> MWHYTSINNDTRVALDPKPNQIRTITKPNTVPQLGTDYLYTFNSQRRSHTLRLLGPFQYFNFSETDRGHPLFRLPLKYPSKAIPADELIDNLHSWMRSVHLLHVRSEDNTLRYNWMLGVYARSTNYTTPVGQLVVNAPAILNYSNPQDAFNSVFVALGIDYIDIPITNSNIFDDSSTPYNVRIWHAPTMTEVNHILALMRKSTLVSTHSSWHWNVLHTFHYRSESDMIDHFAAKILEDWRQKEKLDKGALVEADRVIQRLIPLSSSTYVQRLAAIGALYPNEFTENVLDLSRLSTALLQLSDTYYQHANDQLRRLYRRMYNDSRTLYMTQRHQELLLAQITADPNILLYPYTYIFTTIPTSMNYISNTGQGRIKHSLTVTGATEHDTVADIVLGQTGEDVITISMVEPMSIAVEDMYGYVLDTPTRDIWPADEQIEQKGDAVALYDTKTSRALGMFNNTVRIDDLLSPLLSLVYRTYIKGDTMTMTQGSLDHLTLCAAVDSDITFVGNRMIAPLPEGYIPKPMHRNNSTMKMLSLYVALKKLENFATNSYLMAPDTSIILLGAEREPAVNILRRFNRNVSNVRIIGMGDRAVEPNIRVRVPFPIDKNISADFIICDINSYEDQSFESMFSETISVVTTCASAATRALVKINHPSEYMINSVIERLSQLGGVFYHTALLKTASQNPYSYETYIYITPIAAAVRFPFYSNSAMINRYMTAVADDEMPIIPSIHTVIKGHSNTYSPGLFCGCVDVQSAPLALSQLKSYCSEATTWRVDSDDNLVNIIARIDPARIALEFRTRSNTSAYHEYQRYVPNGLGFKVRKTREFRYMHREVTFIHKLMMYALIREQISLTENMTQVVSIGGRNLADISVVPLNMKYVVIDPATRIETLTQEKKNIEVQSRPFQFDAANMDLENNSIYLFIAVIMNEPNGAATPARMQMDKIRNVATAMLTRTNCVAYISFYEAGIITRLDQSTAHKTIRVEEGRLKVANYVPVDTLVEADVTLMLRDIGITHEIIRPSTPELIDACSNYGIRLGSTGGAVLDVFNHYSPVIKLVRS;>MHSTNNNSNKRNNEEKHKQPEIDSSANNGEGTSGTRAQTVGDTATEAGVRNETEAGASTRRQTDGTGLSGTNAKIATASSARQADVEKPADVTFTIENVDDVGIMQQKKPPTVVQSRTDVFNEQFANEALHPTTKVIFNGLDVNTEVQPLSDDFKQISDPKGYLTYSVKYEDQFTKKDKLRASEADDRIVGPTVNLFKYGAAVVNIDLNRDFFDTATGIDLTKGIPLVQDLLVPIGVTAGAEQSAEYVSGLLMVLFKVMTDNRLVIVGETTTPMSNTLSTVVNNVLRTTYHNNVGVNPALLRDFTQVNWLNRDITNMLQQAGTKYGLGLTETRLDYVRLVKTIVGHALNIDHFAASVLNINLRALMEANVTADDRIKALQAHSMISTQFHGPNQGALRPELAFDHDHIIRCLMLAAANYPRLEGIIVQINTGYVASANVIRPVSEKRYFPENLEQNQSAARLVSAVKARASEADISSIHLAIAREVSPMFNVHELKKIAESFEDPSSIVVVLEFILFALFFPTEFNRIKGDIQNVLLLFFSRWYPVEYGIFVQRGATYTINAAGEFEFSGRNEKWDQALYLSEHFPALFSDVPLAGANTIIAIMRLFTPQGFLRTDDLAIAANFPRASRNPQTYIPYTNQRGTVTNEFASRFRTIVATLANVVNERAVQDDMQKATRSCTKQWLRHLETQFDNIAVAHTDHLSVVYATMSNFMLNFTNNFSGNHATFKPDQYVITSPEGSYKPIIERQGETVDGLTIIDTSIVWPILCQCTYPLVRQSGKGVDAVSIMEEIVYPDPSTTLSQSLSVAQVLSKLTLPDAFINMILSGGDSVVMRTYQTEADDDLDEGIRMTTYDQYLSHIRERLHITNVPDPIYITGASTPDQIAASVQATHVAVVLYQSGVINGPASTYLRENEVLVVMPDYYDVVSRFANANLQMNNNRYHESVLEIADIFDQADFIQTSDAVRQLRALMPTLSTSQIRHAIERIAQITDVDSTDYGKLTLRFLGTLTRSLKMQNAQIRRIRPDGTVLRYDDQIDIEAFRWSRYFLDELQLRRLSVGLRLITNPRIARRFNGVRIMYLTDDDPDPDFVPDVPEGYVAVQYAHRLFSSSLANKRNRVTYTHPPTGMAYPSPTGRPHVHMTINERAGMSKLVADNIIASVIKSNWVVDILDIEYTAEVMTPSEGYTQHVDAESIMTAPKGKLFHLQFMDGLLRPEPSAFDPPASGEDMRLIYPLQPISVARSMRAIVNHNEVDRPRGAVAPSSYEMDTGTLSRNGDLLYSPVANGQVGIPKLEVDHISFSNVVSMMTANIRTGDDMAVERVNPDDVRAINIRNA[2x];>MLQQPTGGYTTLEQFAFTIRNDGTNATPTQFLQLLSYEATENELVKKTIPTPETHLPSARNVPGNVYIEDAITQALFGISAQNVNAHGYFSRLSALALPNTSARLGLDGVIYNSETINIPFYDPAAVANFAATYAKLGNASTPRYRADMIDIYAHVGLELAGTDAERAAGVMPVKRAKFDSWEGSLISLSRDVVNWKILAFLIDLCSLEGEALRAFKTRNRDVFRMMLFIMSTAVAANVVNRKVTKRVDRVLEYIGVNSMRTAGRTATITYDLSRHEFAAKFLQLTFTRWNAASAMIRSMPDMHTPRTSITPAGENALVR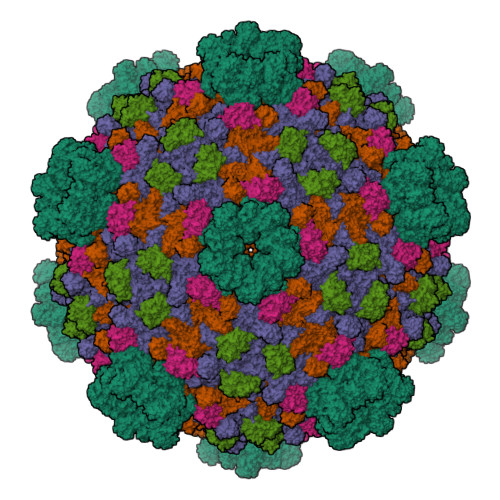HNRYMTENFKGLSPIALAQKKHEMMLHTHEIHSMDIDGSIKNMVERETVNKMNEIDAMNTAPWTEEFAEVEPTTVYERHQIGTDPEQTQLISQDAAVIVHQASSDVDENEYGNSVSELTIDTQSDSVL[2x]>[8x]GSHMKETKKAGPIELPEELEAQRQRHNDPRRPPWPLLHQRVVLLREGKGAPEDIALMWEQTKHYYPADWLIPLELTQVLKYSSGKYLQTYVADPDEMRKE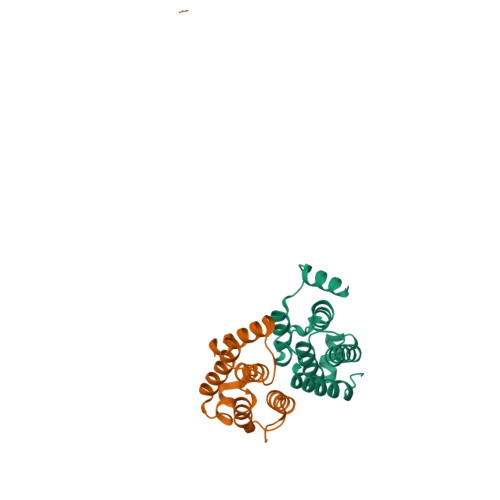VLMQLLNVKYGRVSDPNGGRVNKDVEEIISMAVDDLENMDLNPAADAVLIPTHT>MHHHHHHAQKIVRVGDIQIGNDLPFVLFGGMNVLESRDLAMQVCEEYVRVTEKLGIPYVFKASFDKANRSSIHSFRGPGLEEGMKIFEEIKKTFKVPVITDVHEPFQAQPVAEVCDIIQLPAFLSRQTDLVVAMARTNAVINIKKAQFLAPQEMKHILTKCEEAGNDRLILCERGSSFGYNNLVVDMLGFGIMKQFEYPVFFDVTHALQMPGGRADSAGGRRAQVTDLAKAGLSQKLAGLFLEAHPDPEHAKCDGPCALRLNKLE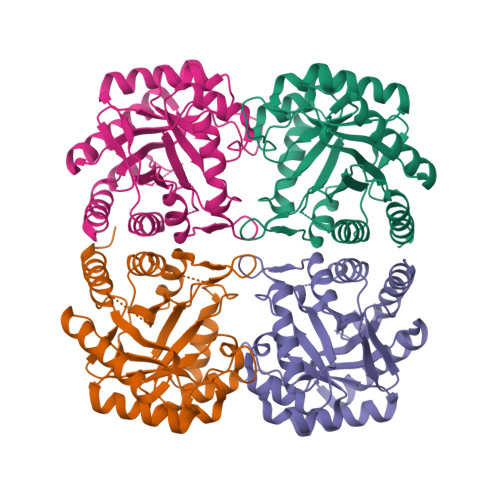AFLSQLKQLDELIKSFPAIETA[4x]7-hydroxy-8-[(E)-phenyldiazenyl]naphthalene-1,3-disulfonic 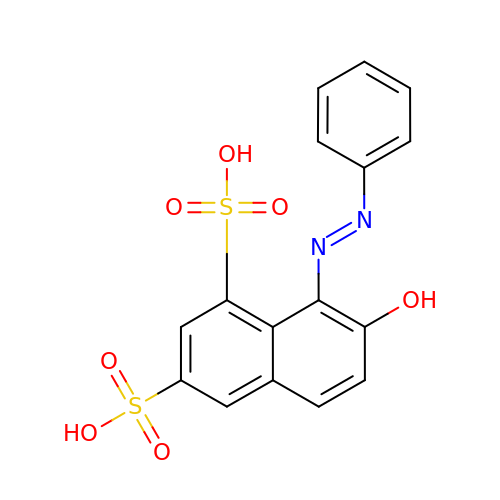acid | C16 H12 N2 O7 S2 | MPVDXIMFBOLMNW-ISLYRVAYSA-N> DERDRVQKKTFTKWVNKHLMKVRKHINDLYEDLRDGHNLISLLEVLSGIKLPREKGRMRFHRLQNVQIALDFLKQRQVKLVNIRNDDITDGNPKLTLGLIWTIILHFQISDIYISGESGDMSAKEKLLLWTQKVTAGYTGIKCTNFSSCWSDGKMFNALIHRYRPDLVDMERVQIQSNRENLEQAFEVAERLGVTRLLDAEDVDVPSPDEKSVITYVSSIYDAFPKVPEGGEGISATEVDSRWQEYQSRVDSLIPWIKQHTILMSDKTFPQNPVELKALYNQYIHFKETEILAKEREKGRIEELYKLLEVWIEFGRIKLPQGYHPNDVEEEWGKLIIEMLEREKSLRP

Evolutionarily conserved in multicellular organisms, spectraplakin proteins such as ACF7 (Actin-Crosslinking Factor 7) can crosslink microtubules and F-actin56. ACF7 harbours an actin-binding domain (ABD) at its N terminus and a microtubule-binding domain at its C terminus. The ABD of ACF7 contains two consecutive CH (calponin homology) domains. ACF7 is a microtubule and F-actin crosslinker that is critically involved in regulation of cell/ECM adhesion dynamics.

To illuminate the potential mechanisms of how F-actin binding of ACF7-CH domains is regulated, we resolved crystal structure of ACF7-NT (containing the CH domains and a part of the plakin domain) at 2.6 Å resolution. ACF7-NT is folded into an elongated polypeptide that is ∼92.4-Å long and ∼58/14.3-Å wide with two tandem CH domains following the spectrin repeat 1 (SR1) of the plakin domain. The SR1 of ACF7’s plakin domain consists of three α-helices connected by short loops that pack in a left-handed helical bundle with a typical up–down–up topology, which is highly conserved among plakin family protein. ACF7’s ABD consists of only α-helices connected by short-loop sequences, and adopts a closed conformation with extensive intramolecular contacts between the two tandem CH domains. Previous biochemical and mutagenesis studies have revealed three major F-ABSs (ABS1–3) in the tandem CH domains, which are conserved in ACF7. However, in closed conformation of ACF7’s ABD, a number of key residues in the ABSs were buried within the protein and were unlikely to be involved in association with F-actin. Interestingly, tyrosine 259 is outside of the conserved ABSs and located at the C-terminal end of the last α-helix in the second CH2 domain. This residue is in close proximity with the hinge region of ABD in the closed conformation. Structural analysis demonstrated that tyrosine 259 forms hydrogen bonds with isoleucine 150 and tyrosine 151 in the hinge region of CH domains. In addition, the hinge region between CH1 and CH2 domain is stabilized by the hydrophobic interactions between isoleucine 150, isoleucine 152 and leucine 165, leucine 167 and tryptophan 168.> FCLTLRRRYTMAHHHHHHENLYFQGMACQVDNPPKTYPNDKTAEYEKYANYMNYLYYYQN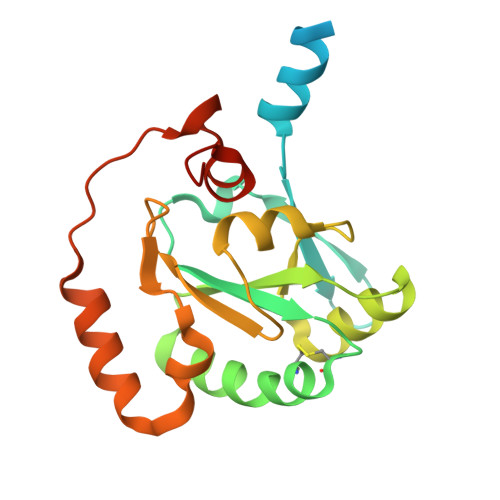NELKKIDSSYFKDKYLGLFFGASWCKYCVTFIDSLNIFKKNFPNVEIIYIPFDRTYQEYQSFLKNTNFYALPFDNYLYICKKYQIKNLPSFMLITPNNNILVKDAAQLIKTDEYINNLKSLIKNYIIHPKTFQFNNRFFDLFRNLEHHHHHH>[2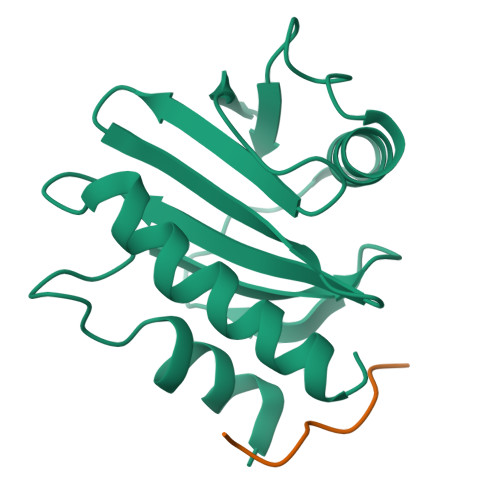x]MSWQSYVDDHLMCEVEGNHLTHAAIFGQDGSVWAQSSAFPQLKPAEIAGINKDFEEAGHLAPTGLFLGGEKYMVVQGEAGAVIRGKKGPGGVTIKKTTQALVFGIYDEPMTGGQCNLVVERLGDYLIESGL;>RVPPPPPPPPPLP[2x]>[2x]GSMEPAMEPETLEARINRATNPLNKELDWASINGFCEQLNEDFEGPPLATRLLAHKIQSPQEWEAI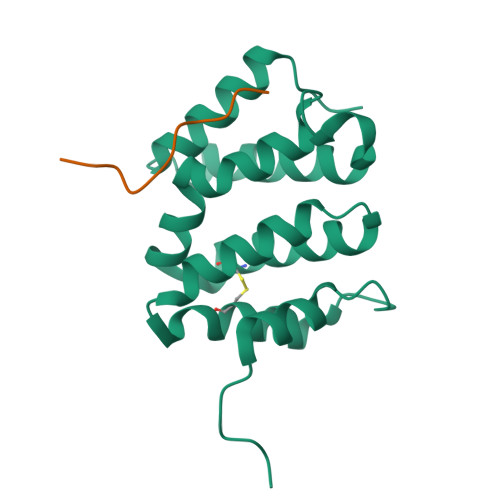QALTVLETCMKSCGKRFHDEVGKFRFLNELIKVVSPKYLGSRTSEKVKNKILELLYSWTVGLPEEVKIAEAYQMLKKQGIVKS;>[2x]ITGFSDDVPMVIA Here we report the mechanism of three Fe(II)/α-ketoglutarate-dependent dioxygenases in bicyclomycin synthesis, which depicts the natural tactic to sequentially hydroxylate specific C−H bonds of similar substrates (cyclodipeptides). Three αKGDs (BcmE/BcmC/BcmG) catalyze site- and stereo-selective hydroxylation of inert C−H bonds in BCM’s (bicyclomycin) cyclic dipeptide scaffold (Fig. 1b3), one of the simplest peptide derivatives without additional functional groups. Our hypothesis posits distinct regulatory mechanisms: BcmE employs steric hindrance, BcmC relies on inherent reactivity, while BcmG utilizes a directing group to control C–H hydroxylation. Although these three enzymes share only 35–42% amino acid identities, the overall structures are similar, and r.m.s.d. values are 0.70 Å (SsBcmE vs SsBcmC), 1.07 Å (SsBcmE vs PaBcmG) and 0.87 Å (SsBcmC vs PaBcmG), respectively.

The DKP ring of substrate 2 is locked in the hydrophobic cavity formed by F245, F276 and F288. Two carbonyl groups of the DKP ring are involved in the formation of direct hydrogen bonds with the imino group of W281 and the water-mediated hydrogen bonds with the amide group of N277, respectively. Steric interaction between W149 and Ile moiety of 2 causes the 7-OH of 2 to move upward, forming a hydrogen bond with T170 at a distance of 2.7 Å. Notably, the distance between C-3’ and the iron center (5.0 Å) seems closer than that of C-2’ (5.7 Å), which contradicts the hydroxylation selectivity of BcmC. We speculated that the crystal structure only captured one state of 2, and the single C-1’ − C-2’ bond of 2 is rotatable which could rotate to the state that C-2’ directs to the iron center, facilitating the hydroxylation reaction. This is in agreement with the results of DFT and MD calculations. However, the single-site mutations of F245A, F276A and F288A have almost no effect on the activity and selectivity, probably because the cavity of the SoBcmC is too large to affect the substrate binding and orientation (volume of SoBcmC is 252 Å3, but that of SsBcmE and PaBcmG are 139 Å3 and 210 Å3, respectively). The W149A mutation dramatically reduces the activity, owing to W149 may lock the substrate in the active pocket. In addition, mutagenesis of T170, N277 and W281, which constituted the hydrogen bond network with substrate 2, resulted in the reduction of C-2’ hydroxylation activity (19%–75% conversion yields) but performed the C-5 hydroxylation activity (4%–23% conversion yields) to generate product 2a, which is also the inherently more reactive site with the lowest activation free energy. Consequently, these findings suggest that the site selectivity of BcmC-catalyzed hydroxylation mainly depends on the innate selectivity of substrate 2, in which one C − H bond is inherently more reactive than the other bonds.

>[4x]HMTTKEMTLQRARTASGELVFETGGGLSQALQDGCFYLAIPEDIDLEPGKLLCRQFYRPAHPGSPELRPYRGFRRNDGIYFDREYYQTEHILADGPAREKYLPPDVVALCERMTSLALLVLTSTLTGLGIDEAVWEKVTGGAVGGGGTQWFAASHYRPERHQLGCAPHKDTGFVTVLYIEQDGLESSVGGEWIPIAPLPGYFLVNFGGATELLTARMGRPVQAILHRVRSCVTEPAREDRFSFAVFANPPATGDLYQMSESGEPVAVRGVEEFLRDFNNETWSDRHTDFGITTTAPGEVHDLEHHHHHHHH> MLETNCLDLRTKLQDLEVANQTLKDEYDALQITFTALEEKLRKT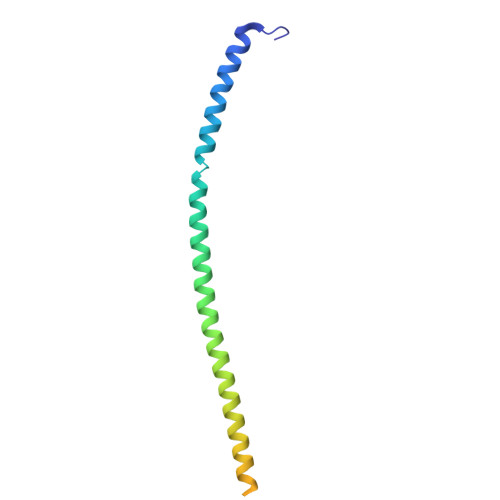TEENQELVTRWMAEKAQEANRLNAENEKDSRRRQARLQKELAEAAKEPLPVEQDDDIEVIVDETSDHTEETSPVRAVSRAAT>GSHMGHWSQGLKISMQDPKMQVYKDEQVVVIKDKYPKARYHWLVLPWTSISSLKAVAREHLELLKHMHTVGEKVIVDFAGSSKLRFRMGYHAIPSMSHVHLHVISQDFDSPCLKNKKHWNSFNTEYFLESQAVIEMVQEAGRVTVRDGMPELLKLPLRCHECQQLLPSIPQLKEH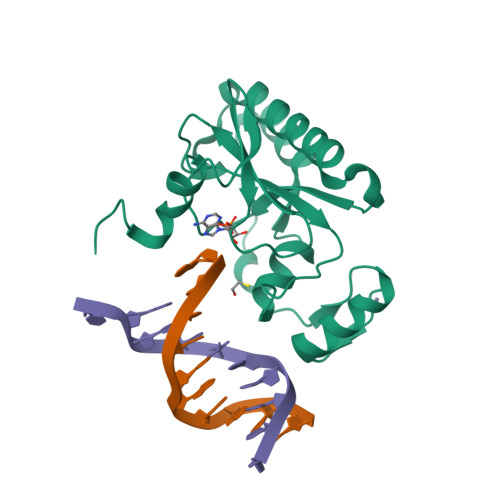LRKHWTQ[2x]> MDGSGEQPRGGGPTSSEQIMKTGALLLQGFIQDRAGRMGGEAPELALDPVPQDASTKKLSESLKRIGDELDSNMELQRMIAAVDTDSPREVFFRVAADMFSDGNFNWGRVVALFYFASKLVLKALSTKVPELIRTIMGWTLDFLRERLLGWIQDQGGWDGLLSYFGTPTW;> SESQEDIIRNIARHLAQVGDSMDRSIPPGLVNGL

The intrinsic pathway to apoptosis is regulated by interactions between members of three factions of the Bcl-2 protein family: the BH3-only proteins such as Bim and Bid, which initiate the process, the essential effectors Bax and Bak, and the prosurvival members, which oppose the action of both other factions. Unlike Bak, which is constitutively anchored in the mitochondrial outer membrane (MOM) via its C-terminal segment, Bax is largely cytosolic in healthy cells and accumulates at the MOM only upon a death signal. Core/latch dimers of Bax and Bak form on treatment of the monomeric proteins with certain BH3 peptides and CHAPS, and Bax and Bak core domains form symmetric homodimers, supporting that unlatching the core domain is a necessary step to Bax and Bak oligomerisation and permeabilisation of the MOM. Bim and Bid are both potent direct activators of Bax, but Bim is less dependent on interactions via its ‘h0' residues than is Bid.

Earlier work had demonstrated that BidBH3 M97 contacts Bax I66, and alanine mutants at either or both of these positions reduced the capacity of the peptide to release the core domain from the latch domain. α2 in equivalent complexes, we crystallised a core/latch dimer complex of BaxI66AΔC21 with BidBH3. That structure is very similar to the wild-type complex, the largest difference being that the C terminus of the Bid peptide is disordered in the crystal, rather than folding back over Bax I66A as it does with Bax I66. In addition, a slight ‘collapse' of Bax α2 towards the core of the complex is evident in a 1 Å shortening of the distance between the Cα atoms of Bid M97 and Bax I66A (8.2 Å) as compared with Bax I66 (9.3 Å). As a consequence, the cavity in the BidBH3:BaxI66AΔC21 structure is reduced to a size not significantly larger than cavities found (for example) in the interior of the complex between BimBH3 and Bcl-xL.> MSEKTTKGVQLLRGDPKKAIVRLSIPMMIGMSVQTLYNLADGIWVSGLGPESLAAVGLFFPVFMGIIALAAGLGVGTSSAIARRIGARDKEGADNVAVHSLILSLILGVTITITMLPAI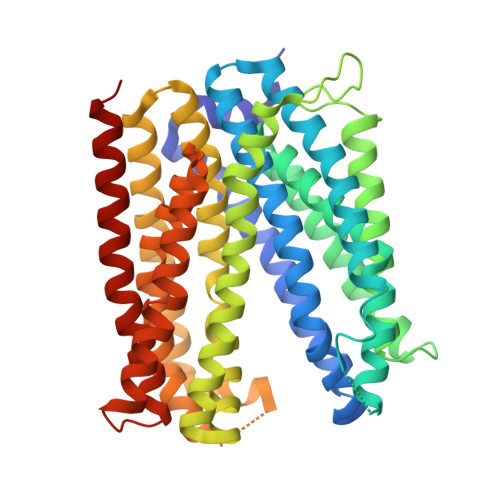DSLFRSMGAKGEAVELAIEYARVLLAGAFIIVFNNVGNGILRGEGDANRAMLAMVLGSGLNIVLDPIFIYTLGFGVVGAAYATLLSMVVTSLFIAYWLFVKRDTYVDITLRDFSPSREILKDILRVGLPSSLSQLSMSIAMFFLNSVAITAGGENGVAVFTSAWRITMLGIVPILGMAAATTSVTGAAYGERNVEKLETAYLYAIKIAFMIELAVVAFIMLFAPQVAYLFTYSESAQVIKGDLISALRTLPVFLVLTPFGMMTSAMFQGIGEGEKSLILTIFRTLVMQVGFAYIFVHYTTLGLRGVWIGIVIGNMVAAIVGFLWGRMRISALKKTSATGGKR>[4x]MTGDCMPVLVLMAAVLTVTGAVPVARLRGALPDARGCHIAQFKSLSPQELQAFKRAKDALEESLLLKDCKCRSRLFPRTWDLRQLQVRERPVA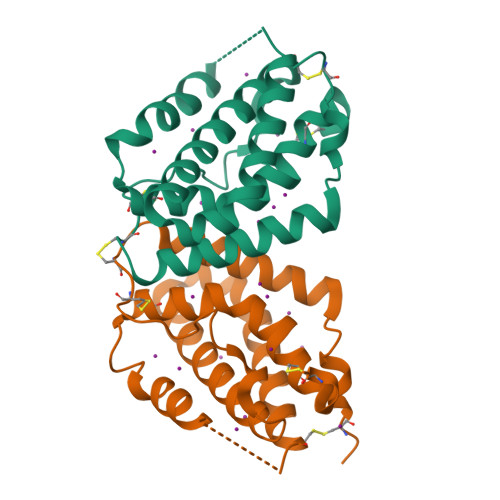LEAELALTLKVLEATADTDPALGDVLDQPLHTLHHILSQLRACIQPQPTAGPRTRGRLHHWLHRLQEAPKKESPGCLEASVTFNLFRLLTRDLNCVASGDLCV> YNQNDALPQM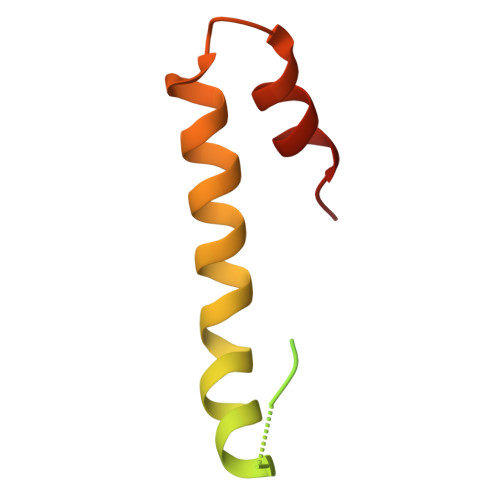AQQGTTPQIALPQVKGPAVLAGYSEEQGAPQVITNSSSSDTRWHEQRLPIYLRQHVQQSAVSGTESALPYARAASLENR> GAGCAGCCTXTACGGACA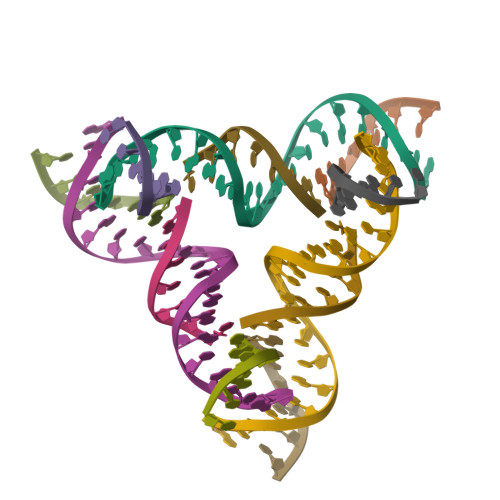TCA;> CCGTAXA;> GGCTGCT;> CTGATGT> SRANDAPIVLLHGFTGWGREEMFGFKYWGGVRGDIEQWLNDNGYRTYTLAVGPLSSNWDRACEAYAQLVGGTVDYGAAHAAKHGHARFGRTYPGLLPELKRGGRIHIIAHSQGGQTARMLVSLLENGSQEEREYAKAHNVSLSPLFEGGHHFVLSVTTIATPHDGTTLVNMVDFTDRFFDLQKAVLKAAAVASNVPYTSQVYDFKLDQWGLRRQPGESFDQYFERLKRSPVWTSTDTARYDLSVPGACKLNQWVKASPNTYYLSFATERTYRGALTGNYYPELGMNAFSAVVCAPFLGSYRNATLGIDDRWLENDGIVNAFSMNGPKRCSTDRIVPYDGTIKKGVWNDMGTYNVDHLEVIGVDPNPLFDIRAFYLRLAEQLA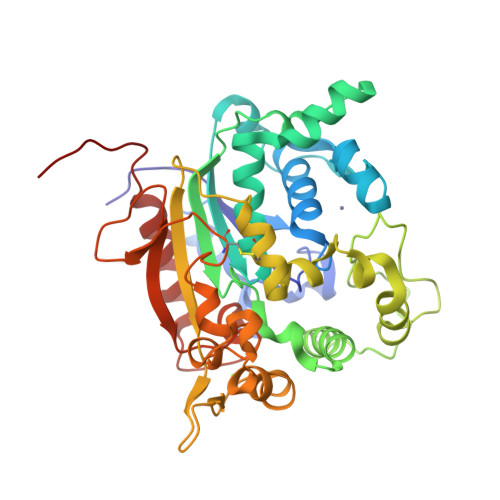SLQPHHHHHH> SNAMDGQQLNRLLLEWIGAWDPFGLGKDAY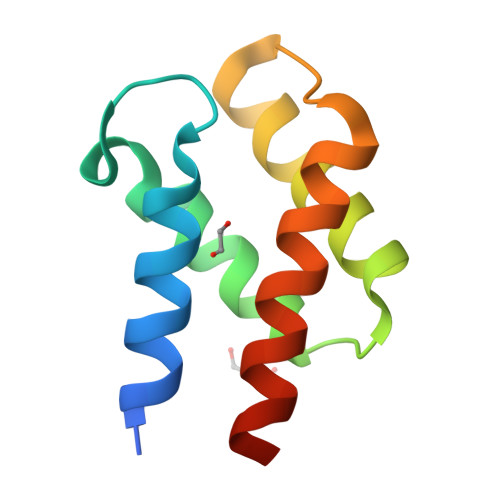DVEAASVLQAVYETEDARTLAARIQSIYEFAFDEPIPFPHCLKLARRLLELKQAASCPLP>[4x]MTPSHPARPSRSGILVFDVNETLLDLTS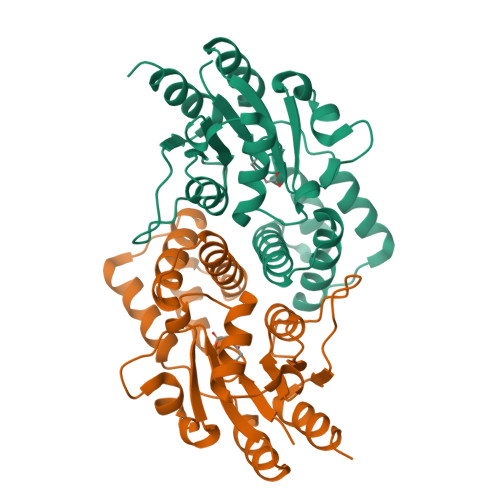LSPLFERVFGDAKVLREWFPELILYSQTLTLTGLYRPFGEIAAAVFEMVAANHQAKVTPDDIAELKTRLTSMPAYPDVAPALTRLQDAGFRLVTLTNSAPSPAPSPLEKAGIASFFEAHLTVHSSQRFKPHPSVYDSTAETLGAKPEELCMIACHIWNTIGAQARGWRGGFVARPHNTPLTLAEVPQPDFIGRDMGELADQLIASLTA2-(4-(2-((3-(5-(PYRIDIN-2-YLTHIO)THIAZOL-2-YL)UREIDO)METHYL)-1H-IMIDAZOL-4-YL)PHENOXY)ACETIC 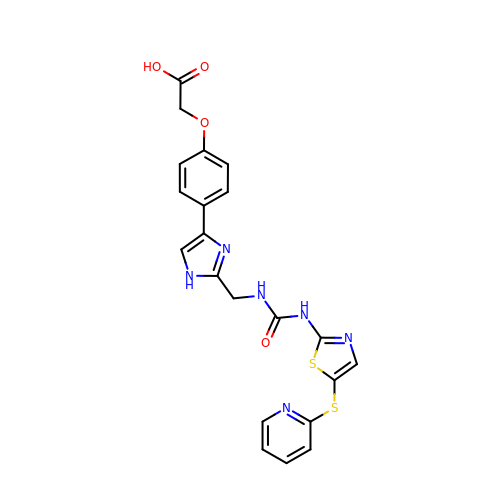ACID | C21 H18 N6 O4 S2 | SSXCWVOQWRUMGN-UHFFFAOYSA-N>MHVIKRDGRQERVMFDKITSRIQKLCYGLNMDFVDPAQITMKVIQGLYSGVTTVELDTLAAETAATLTTKHPDYAILAARIAVSNLHKETKKVFSDVMEDLYNYINPHNGKHSPMVAKSTLDIVLANKDRLNSAIIYDRDFSYNYFGFKTLERSYLLKINGKVAERPQHMLMRVSVGIHKEDIDAAIETYNLLSERWFTHASPTLFNAGTNRPQLSSCFLLSMKDDSIEGIYDTLKQCALISKSAGGIGVAVSCIRATGSYIAGTNGNSNGLVPMLRVYNNTARYVDQGGNKRPGAFAIYLEPWHLDIFEFLDLKKNTGKEEQRARDLFFALWIPDLFMKRVETNQDWSLMCPNECPGLDEVWGEEFEKLYASYEKQGRVRKVVKAQQLWYAIIESQTETGTPYMLYKDSCNRKSNQQNLGTIKCSNLCTEIVEYTSKDEVAVCNLASLALNMYVTSEHTYDFKKLAEVTKVVVRNLNKIIDINYYPVPEACLSNKRHRPIGIGVQGLADAFILMRYPFESAEAQLLNKQIFETIYYGALEASCDLAKEQGPY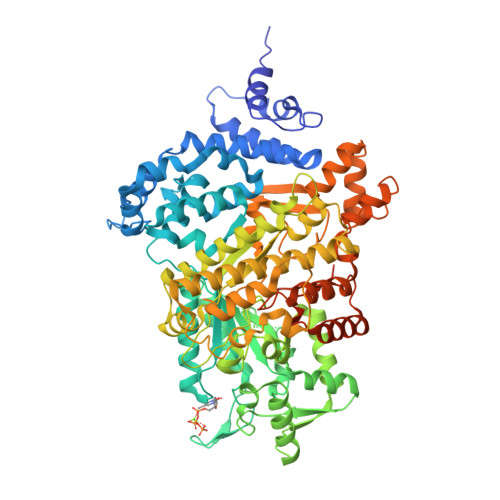ETYEGSPVSKGILQYDMWNVTPTDLWDWKVLKEKIAKYGIRNSLLIAPMPTASTAQILGNNESIEPYTSNIYTRRVLSGEFQIVNPHLLKDLTERGLWHEEMKNQIIACNGSIQSIPEIPDDLKQLYKTVWEISQKTVLKMAAERGAFIDQSQSLNIHIAEPNYGKLTSMHFYGWKQGLKTGMYYLRTRPAANPIQFTLNKEKLKDKEKVSKEEEEKERNTAAMVCSLENRDECLMCGS[2x]GLIC is a bacterial homologue of the pentameric ligand-gated ion channels (pLGICs) that mediate the fast chemical neurotransmission of nerve signalling in eukaryotes. Because the activation and allosteric modulation features are conserved among prokaryotic and eukaryotic pLGICs, GLIC is commonly used as a model to study the allosteric transition and structural pharmacology of pLGICs. Unlike the other pLGICs, GLIC displays a particular activation mechanism in which protons, rather than a sizable agonist, trigger ion-channel opening. Here, experimental evidence for carboxylate binding to GLIC is provided by solving its X-ray structures with a series of monocarboxylate and dicarboxylate derivatives, and two carboxylate-binding sites are described: (i) the ‘intersubunit’ site that partially overlaps the canonical pLGIC orthosteric site and (ii) the ‘intrasubunit’ vestibular site, which is only occupied by a subset of the described derivatives.

We thus aimed to check whether dicarboxylic acids are also able to bind GLIC similarly to monocarboxylates. A 2.5 Å resolution structure was obtained from crystals grown in a solution buffered at pH 4.0 using 0.1 M succinate (diC4). In this structure, two identical GLIC pentamers were found in the asymmetric unit, with a c unit-cell parameter that was twice as large as in the other structures described in this study. The succinate molecule bound in the intersubunit site is modelled with one of its carboxylate moieties superimposed on the position of acetate below Loop C. This carboxylate moiety interacts with the side chains of residues from two adjacent subunits: Arg77 (Loop A) and Glu181 (Loop C) from one subunit and Arg105 from the neighbouring subunit. The succinate molecule in the intrasubunit site displayed a higher flexibility than the intersubunit succinate, as seen in the different subunits. Indeed, the first succinate carboxylic moiety binds in the same way (in all subunits) as acetate: through a hydrogen bond to the hydroxyl group of the well conserved Tyr102 and a salt bridge to the guanidinium group of Arg85, which itself makes a salt bridge with Glu104. However, the second carboxylic moiety of the intrasubunit succinate molecule only interacts with the main-chain carbonyl group of Pro74, leading to different binding poses of succinate in the intrasubunit site in the different subunits. Unlike the intersubunit succinate, where both carboxylic groups are tightly coordinated through hydrogen bonds to Arg85, Tyr102 and Glu104, the second carboxylic group of succinate in the intrasubunit site points almost freely towards the solvent and is only loosely coordinated through a hydrogen bond to the main chain of Pro74 in most of the modelled succinate poses.

>[10x]GQDMVSPPPPIADEPLTVNTGIYLIECYSLDDKAETFKVNAFLSLSWKDRRLAFDPVRSGVRVKTYEPEAIWIPEIRFVNVENARDADVVDISVSPDGTVQYLERFSARVLSPLDFRRYPFDSQTLHIYLIVRSVDTRNIVLAVDLEKVGKNDDVFLTGWDIESFTAVVKPANFALEDRLESKLDYQLRISRQYFSYIPNIILPMLFILFISWTAFWSTSYEANVTLVVSTLIAHIAFNILVETNLPKTPYMTYTGAIIFMIYLFYFVAVIEVTVQHYLKVESQPARAASITRASRIAFPVVFLLANIILAFLFFGF> KVGVIVGAEQQVAEVAQKVAKDKYGLDVELVTFNDYVLPNEALSKGDID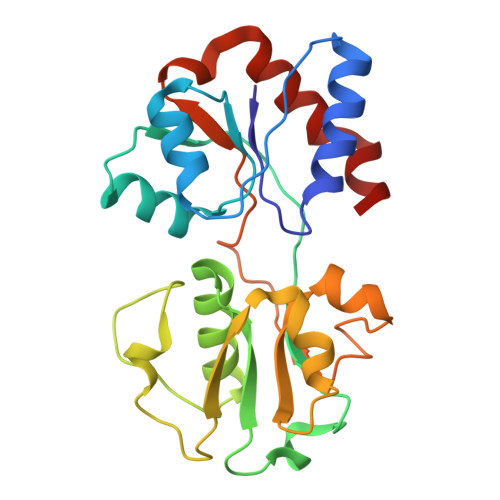ANAFQHKPYLDQQLKDRGYKLVAVGNTFVYPIAGYSKKIKSLDELQDGSQVAVPNDPTNLGRSLLLLQKVGLIKLKDGVGLLPTVLDVVENPKNLKIVELEAPQLPRSLDDAQIALAVINTTYASQIGLTPAKDGIFVEDKESPYVALIVTREDNKDAENVKKFVQAYQSDEVYEAA> MRVIVFFDLPVITPENRHNYSVFRKYLIKSGFIMQQKSVY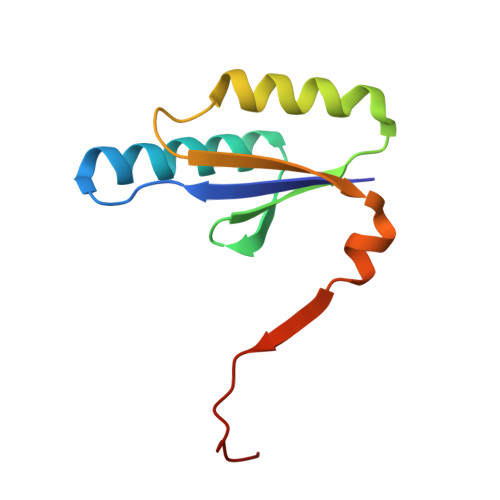SKLVLNLTNRDSIVKSIEKNKPPEGLVEVLTVTEKQYAKMEIIIGESKTEYLN> MSLRRGIYHIENAGVPSAIDLKDGSSSDGTPIVGWQFTPDTINWHQLWLAEPIPNVADTFTLCNLFSGTYMDLYNGSSEAGTAVNGWQGTAFTTNPHQLWTIKKSSDGTSYKIQNYGSKTFVDLVNGDSSDGAKIAGWTGTWDEGNPHQKWYFNRMSVSSAEAQAAIARNPHIHGTYRGYILDGEYLVLPNATFTQIWKDSGLPGSKWRE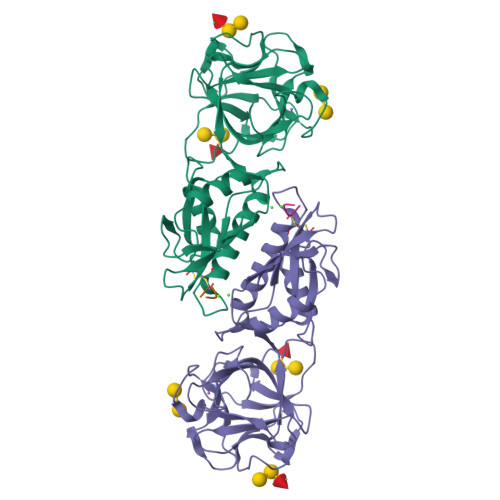QIYDCDDFAIAMKAAVGKWGADSWKANGFAIFCGVMLGVNKAGDAAAAYNFTLTKDHADIVFFEPQNGGYLNDIGYDSYMAFY;> PVPRAHS>[3x]GAMGEITIKLPDSVKVSTNSILYKCGAKDLSVTYYNAGDISLAKLELEDETVV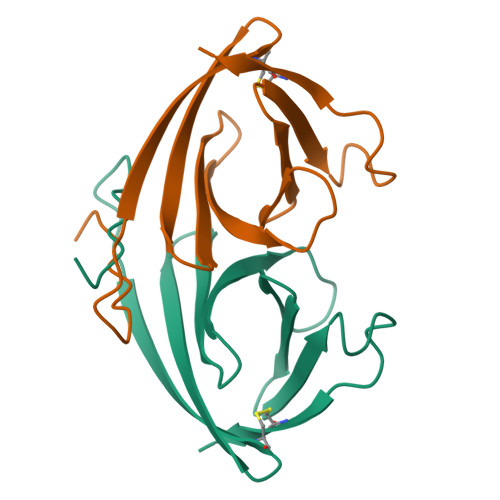ASNVISGSGAKYAGSVYIWWTKGKTASLYNLIDNPEEDKPISCVEQ> GDVEEAIDRAVARVADTMPTGPRNTESVPALTAVETGHTSQVVPGDTMQTRHVKNYHSRTESSIENFLCRAACVYIATYKSAGGTPTERYASWRINTRQMVQLRRKFELFTYLRFDMEITFVITSTQDPGTQLAQDMPVLTHQIMYIPPGGPVPNSATDFAWQSSTNPSIFWTEGCAPARMSVPFISIGNAYSNFYDGWSHFTQEGVYGFNSLNNMGHIYVRHVNEQSLGVSTSTLRVYFKPKHVRAWVPRPPRLSPYVKSSNVNFKPTAVTTERKDINDVGTLR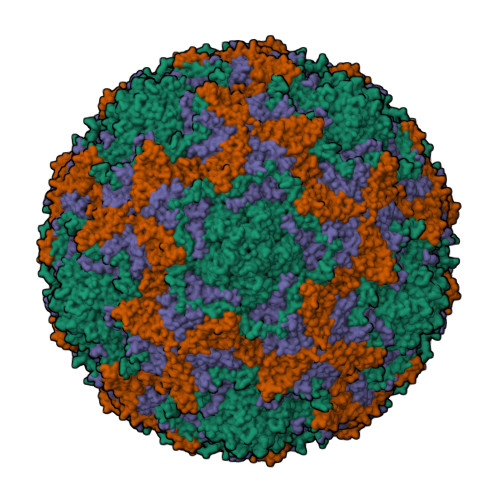PVGYTNH;> GAQVSTQKTGAHETSLTASGNSTIHYTNINYYKDAASNSANRQDFTQDPSKFTEPMKDVMIKSLPALNSPTVEECGFSDRVRSITLGNSTITTQECANVVVGYGVWPSYLQDNEATAEDQPTQPDVATCRFYTLDSIQWQKESDGWWWKFPEALKNMGLFGQNMEYHYLGRSGYTIHVQCNASKFHQGCLLVVCVPEAEMGCSDVEREVVAASLSSEDTAKSFSRTESNGQHTVQTVVYNAGMGVGVGNLTIFPHQWINLRTNNSATIVMPYINSVPMDNMFRHYNFTLMIIPFAKLEYTEQASNYVPITVTVAPMCAEYNGLRLASHQ;> GLPTMLTPGSNQFLTSDDFQSPSAMPQFDVTPEMKIPGEVHNLMEIAEVDSVVPVNNTKENINSMEAYRIPVTGGDQLHTQVFGFQMQPGLNSVFKRTLLGEILNYYAHWSGSVKLTFVFCGSAMATGKFLLAYSPPGASPPQNRKQAMLGTHVIWDVGLQSSCVLCIPWISQTHYRLVQQDEYTSAGYVTCWYQTGLIVPPGAPPSCTILCFASACNDFSVRNLRDTPFIEQTQLLQ>MGESKRTEKTRVLVVGATGYIGKRIVRACLAEGHETYVLQRPEIGLEIEKVQLFLSFKKLGARIVEGSFSDHQSLVSAVKLVDVVVSAMSGVHFRSHNILVQLKLVEAIKEAGNVKRFLPSEFGMDPPRMGHALPPGRETFDQKMEVRQAIEAAGIPYTYVVGACFAAYFAGNLSQMVTLLPPKEKVNIYGDGNVKVVFADEDDIAKYTAKTLNDPRTLNKTVNIRPPDNVLTQLELVQIWEKLTGKELEKTNIAAQDFLANIEQMEIPHQAGIGHFYHIFYEGCLTDHEVGEDEEASSLYPDVKYKRMDDYLRMFL[6x]

Pinoresinol/lariciresinol reductase (PLR), an NADPH-dependent reductase, converts pinoresinol to lariciresinol and subsequently to secoisolariciresinol. Here, we present crystal structures of IiPLR1 from Isatis indigotica and pinoresinol reductases (PrRs) AtPrR1 and AtPrR2 from Arabidopsis thaliana, in the apo, substrate-bound and product-bound states. The crystal structures were captured in the apo, substrate-bound and/or product-bound forms. We found that, for all 16 structures we solved, each enzyme adopts a similar head-to-tail dimer conformation, strongly suggesting that each PLR/PrR functions as a homodimer, consistent with the literature that TpPLR1 exists as a dimeric entity in solution. Each structure contains a head-to-tail homodimer, and the catalytic pocket comprises structural elements from both monomers. β4 loop covers the top of the pocket, and residue 98 from the loop governs catalytic specificity.

In contrast to IiPLR1_NAP_ + PIN, the β4 loops of AtPrR1_NAP_ + PIN and AtPrR2_NAP_ + PIN can be clearly identified. These well-defined loops twist as an “8” shape and cover both the NADP+-binding and substrate-binding grooves. Within the twisted loop, His93 and His97 “grasp” helices α5 and α10, while Val92 and Phe94 interact directly with (+)-pinoresinol; Arg95 strongly interacts with NADP+ as well as each of the GXXGXXG motif and α2-helix from neighboring protomer of the dimer. Similar β4 loops are also observed in all other AtPrR1 substrate/product-bound structures, whereas each β4 loop is disordered in the corresponding IiPLR1 structures, which indicates that the β4 loop may participate in substrate selectivity and, hence, catalysis. Furthermore, Leu46 (corresponding to Val46 in IiPLR1), His276 and Phe277 of AtPrR1 are positioned similar to the corresponding residues of IiPLR1 to effect substrate binding or product release, except that the β4 loops cover the substrate/product, which are disordered in the IiPLR1 structures. Besides the β4 loop, Val46 in IiPLR1 is replaced with Leu46 in AtPrR1, which has the effect of compressing the substrate-binding pocket.>[2x]KFAEHLSAHITPEWRKQYIQYEAFKDMLYSAQDQAPSVEVTDEDTVKRYFAKFEEKFFQTCEKELAKINTFYSEKLAEAQRRFATLQNELQSSLDAQKESTGVTTLRQRRKPVFHLSHEERVQHRNIKDLKLAFSEFYLSLILLQNYQNLNFTGFRKILKKHDKILETSRGADWRVAHVEVAPFYTCKKINQLISETEAVVTNELEDGDRQKAMKRLRVPPLGAAQPAPAWTTFRVGLFCGIFIVLNITLVLAAVFKLETDRSIWPLIRIYRGGFLLIEFLFLLGINTYGWRQAGVNHVLIFELNPRSNLSHQHLFEIAGFLGILWCLSLLACFFAPISVIPTYVYPLALYGFMVFFL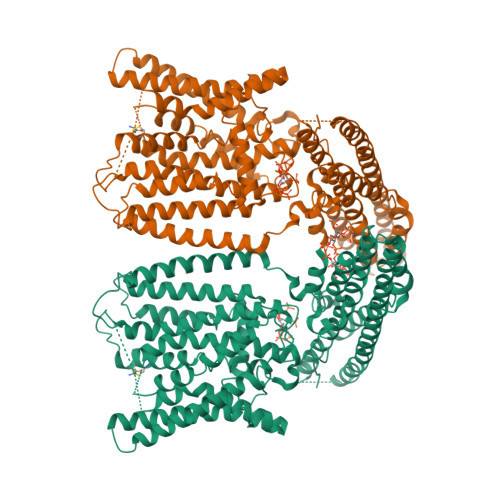INPTKTFYYKSRFWLLKLLFRVFTAPFHKVGFADFWLADQLNSLSVILMDLEYMICFYSLELKWDESKGLLPNNSEESGICHKYTYGVRAIVQCIPAWLRFIQCLRRYRDTKRAFPHLVNAGKYSTTFFMVTFAALYSTHKERGHSDTMVFFYLWIVFYIISSCYTLIWDLKMDWGLFDKNAGENTFLREEIVYPQKAYYYCAIIEDVILRFAWTIQISITSTTLLPHSGDIIATVFAPLEVFRRFVWNFFRLENEHLNNCGEFRAVRDISVA>MGSSHHHHHHENLYFQSNAETVAAIKTLIQQLAQSTDQFGRAEINDALRELQYSLETPFDTVMRMSLDTCQVAVARIGSDLGLFKHLSQCASPQSAEELADHLGCGRELMSRLLRYMASVRMVQQTDDIKYISSNITQTLAVPGLEAGMRHAFENLWPVLMALPDFLAERKYPDIVDAKDTAFQKAFNTDQDCFHWLATQPTRIANFKVLLTDERTPNFLSTFPLEKELGSWSAEPEKALFVDIGGGMGHACIRLREKYPNQPGRVILQDLPPVLQAAQATLPLSGIESMPHNFHTPQPVQGAKFYFLRLILRDFPDHQALEILQNIVPAMDAESRIVIDDGV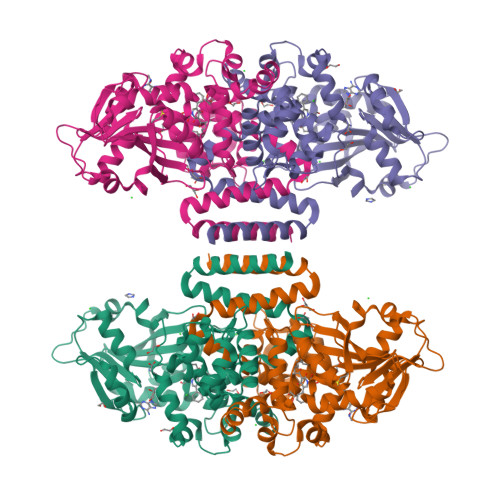PPEKGARWAETGTDICIMSALGSKERTQRQWEELAAKAGLQLQALYQYTWPVVNAAMVFSLQ[2x]4-{2-[(1S)-1-({[trans-4-(aminomethyl)cyclohexyl]carbonyl}amino)-2-phenylethyl]-1H-imidazol-4-yl}benzamide | C26 H31 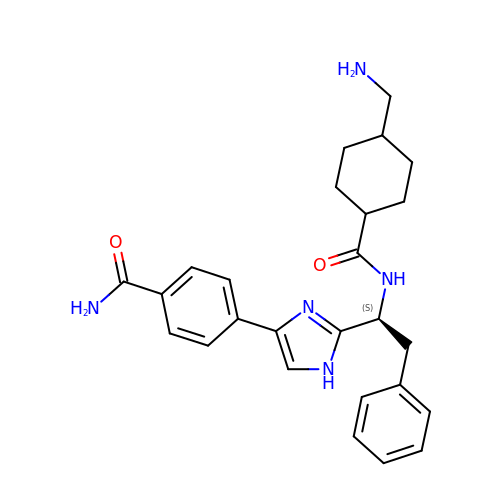N5 O2 | UXCQKLRVLBOFGG-NYVOZVTQSA-N> MHHHHHHHHENLYFQGGSSTAGD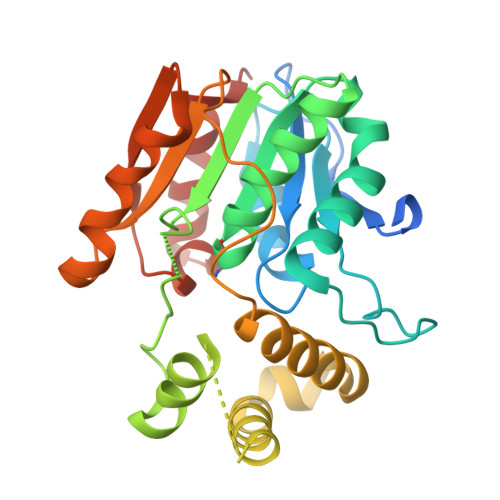PTAKLVRLNPRGGDGPGIVFAPPAGGTVLGYIELARHLKGFGEIHGVEAPGLGAGETPVYPSFEEMVQFCSDSAAGVAGDGVYIGGHALGGHIAFYLATMLLDRGIRPKGLIILDTPPRLGDIPVADADLTEEETKVFILAMGIGGMLDQDRDALKDLPYEEAKQLLLDRAKNDPRVSAFLSEDYLDRFLRLQMHQLMYSRDVVLPQRKLDIPIHVFRTKNHAPEVARLFSAWENYAAGEVTFVDIPGDHATMLRAPHVSEVAQLLDRHCGLPSDDGPRG We report an in silico strategy for the biocatalytic synthesis of chiral N- and O-heterocycles via Baldwin cyclization modes of hydroxy- and amino-substituted epoxides and oxetanes using the limonene epoxide hydrolase from Rhodococcus erythropolis. We turned to cofactor-independent limonene epoxide hydrolases (LEHs) that normally catalyze direct hydrolysis of epoxides by positioning and activating water at the active site. On the basis of the well-documented mechanism of ReLEH, a water molecular is positioned by H-bonds to N55 and Y53 while D132 abstracts a proton from the water, enabling a smooth nucleophilic attack on one of the substrate’s epoxide carbon center. We have rationally engineered the epoxide hydrolase ReLEH with construction of a general platform for Baldwin cyclization reactivity of hydroxy- and amino-epoxides and oxetanes.

After screening 576 transformants with automated gas chromatography (GC) for 95% library coverage, a distinctly improved mutant SZ616 (Y53F/N55A/I116V) was obtained, enabling a 2:3 ratio of 6.7 favoring the Baldwin reaction mode, although conversion to the anti-Baldwin product 3 was only 13%, the rest of complete conversion being. We were pleased to discover that when using triple mutant SZ616 (Y53F/N55A/I116V), the tetrahydrofuran product 10 was obtained in 96% conversion with a 72:28 enantioselectivity ratio (e.r.). In order to gain insights on the active substrate-LEH interactions, the X-ray structures of the key variants SZ612 and SZ616 were analyzed. Consequently, the representative substrates in complex with LEH mutants, including the models SZ612‒(R)-1 and SZ616‒(R)-1, were constructed by molecular docking. Following the docking analysis, the epoxy ring O-atom of the substrate consistently establishes a hydrogen-bond interaction with the protonated catalytically active D101; the aforementioned hydrogen-bond network with water molecular is terminated by substitutions Y53F and N55A, enabling the substrate distal hydroxyl moiety to form a hydrogen-bond interaction with the deprotonated D132. In contrast, the model SZ616‒(R)-1 unveiled two peaks in terms of the dihedral angle θ, revealing that the attack from Si- or Re-face has no preference in the case of SZ616. Moreover, for both of the SZ612 and SZ616 mutants, the slightly shorter distance d1 was observed during the simulations, indicating that the ON atom preferentially attacks C1. Furthermore, to better illustrate the bond forming and breaking in the Baldwin/anti-Baldwin selection pathways, the hybrid QM/MM scheme was employed, enabling the calculation the activation energy barriers. It is of interest to note that the shorter distance d2 allows a relatively low activation energy, and hence the formation of Baldwin product is favored for the two variants.

>MHHHHHHTSKIEQPRWASKDSAAGAASTPDEKIVLEFMDALTSNDAAKLIEYFAEDTMFQAMPLPPAYGRDAVEQTLAGLFTVMSIDAVETFHIGSSNGLVYTERVDVLRALPTGKSYNLSVLGVFQLTEGKITGWRDYFDLREFEEAVDLPLRG[4x]>MAHRSRCNCNDTSNSNGSQHGINLPLRKIDTYDPCVNCRVKPHLCPKPHPCPKPENLEADIVIIGAGAAGCVLAYYLTKFSDLKIILLEAGHTHFNDPVVTDPMGFFGKYNPPNENIRMSQNPSYAWQPALEPDTGAYSMRNVVAHGLAVGGSTAINQLNYIVGGRTVFDNDWPTGWKYDDIKKYFRRVLADISPIRDGTKVNLTNTILESMRVLADQQVSSGVPVDFLINKATGGLPNIEQTYQGAPIVNLNDYEGINSVCGFKSYYVGVNQLSDGSYIRKYAGNTYLNSYYVDSNGFGIGKFSNLRVISDAVVDRIHFEGQRAVSVTYIDKKGNLHSVKVHKEVEICSGSFFTPTILQRSGIGDFSYLSSIGVPDLVYNNPLVGQGLRNHYSPITQVSVTGPDAAAFLSNTAAGPTNMSFRGAGMLGYHKLEPNKPSNAGSVTYRKYELLVTGGVAISADQQYLSGISSSTGNYFALIADDIRFAPVGYIKIGTPNFPRDTPKIFFNTF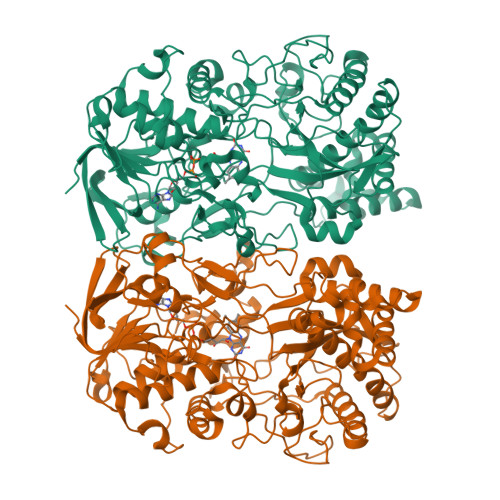VNYTPTTDPADQQWPVAQKTLAPLISALLGYDAIYQIVQQMKVVAVNAGFNVTLQMAYPPNDLLVELHNGLNTYGINWWHYFVPSLVNDDTPAGKLFASTLSKLSYYPRSGAHLDSHQSCSCSIGGTVDTELKVIGVENVRVTDLSAAPHPPGGNTWCTAAMIGARATDLILGKPLVANLPPEDVPVFTTS[2x]> AYVEIIEQPKQRGMRFRYKCEGRSAGSIPGERSTDTTKTHPTIKINGYTGPGTVRISLVTKDPPHRPHPHELVGKDCRDGYYEADLCPDRSIHSFQNLGIQCVKKRDLEQAISQRIQTNNNPFHVPIEEQRGDYDLNAVRLCFQVTVRDPAGRPLLLTPVLSHPIFDNRA;> GAMSHPHDSKVFPDLPEHQDNPSQLRLQHDGLATDDKARLEPMCLAEYLISGPGGMDPDIEIDDDTYDECREVLSRILEDAYTQSGTFRRLMNYAYDQELHDVEQRWLLGAGENFGTTVTDEDLESSEGRKVIALNLDDTDDDSIPEYYESNDGPQQFDTTRSFIHQVVHALTHLQDKEDSNPRGPV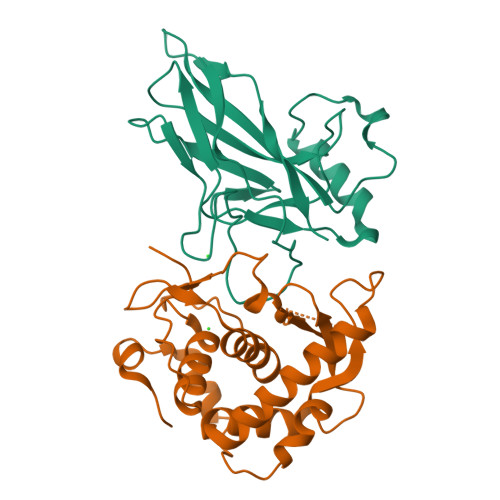VEYTNIILKEMGHTSPPRIAYEFSN> GSMRTEK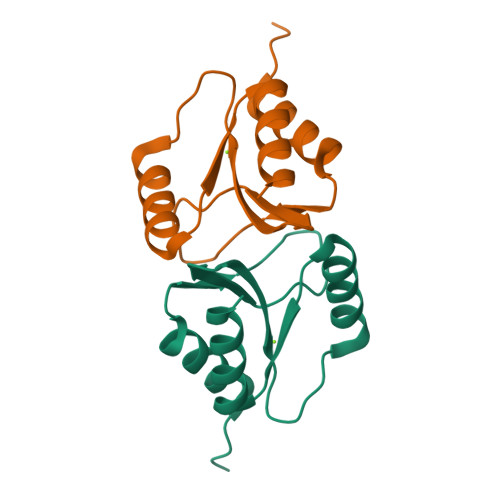DIENYLKKKTKGLCLKFTSPGTIGVPDRIVVMNTGTFFVEVKAPGKKPRPSQVAMHKKIKEAGQHVWVVDSYESVDMALKEMENW> GGGMDTLLILGDSLSAGYRMSASAAWPALL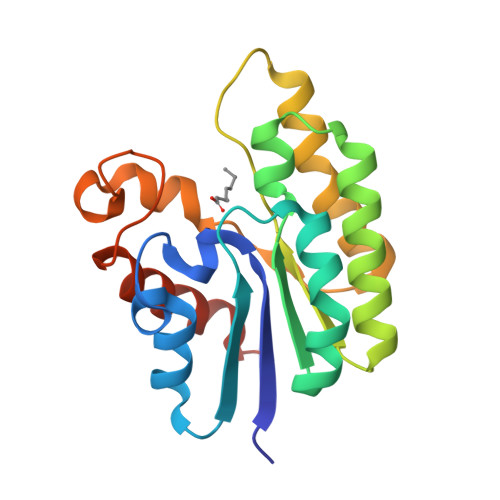NDKWQSKTSVVNASISGDTSQQGLARLPALLKQHQPRWVLVELGGNDGLRGFQPQQTEQTLRQILQDVKAANAEPLLMQIRLPANYGRRYNEAFSAIYPKLAKEFDVPLLPFFLEEVKKKPQWMQDDGIHPNRDAQPFIADWMAKQLQPLVNHDS>AKRKRIEMYTKASFKASNQKIEQIWKTQQEEIQKLNNEYSQQFMNVLQQWELDIQKFEEQGEKLSNLFRQQQKIFQQSRIVQSQRMKAIKQIHEQFIKSLEDVEKNNDNLFTGTQSELKKEMAMLQKKVMMETQQQEMANVR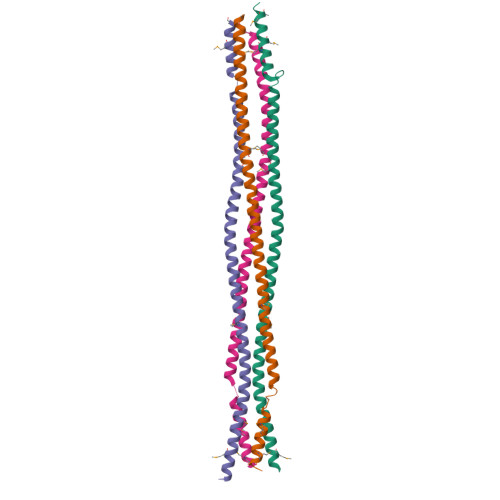KS[4x]4-{[5-chloro-4-(1H-indol-3-yl)pyrimidin-2-yl]amino}-N-ethylpiperidine-1-carboxamide | C20 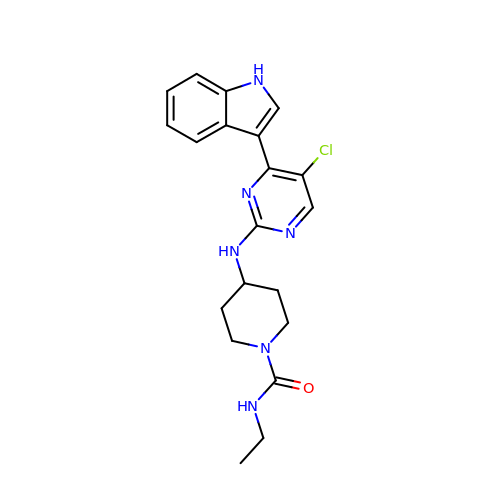H23 Cl N6 O | ARMFMDYRYOKSOW-UHFFFAOYSA-N[4-(3-{[2-chloro-3-(trifluoromethyl)benzyl](2,2-diphenylethyl)amino}propoxy)-1H-indol-1-yl]acetic 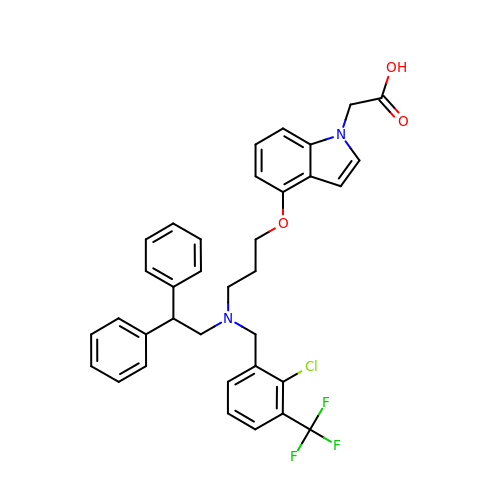acid | C35 H32 Cl F3 N2 O3 | RHWNXOWPCIQOAH-UHFFFAOYSA-N The population density of E. huxleyi is restricted by Nucleocytoviricota viruses, including E. huxleyi virus 201 (EhV-201). Here, we show that the dsDNA genome inside the EhV-201 virion is protected by an inner membrane, capsid, and outer membrane. Virions of coccolithoviruses are unique within the family Phycodnaviridae because they contain not only a membrane inside the capsid but also an additional membrane wrapped around the outer capsid surface, similar to the African swine fever virus from the family Asfaviridae. EhV-201 virions infect E. huxleyi by using fivefold vertices to bind to and fuse the virus’ inner membrane with the cell plasma membrane.

(F) AlphaFold2-predicted structure of EhV-201 major capsid protein with double jelly roll fold. The jellyroll cores J1 and J2 are each composed of two β sheets named according to the convention BIDG and CHEF. The transmembrane proteins from the EhV-201 outer membrane bind to the capsid; however, there are additional interactions between the major capsid proteins and the outer membrane. The loop is predicted to form helices α3 and α4, which are 13- and 20-residue long, respectively, and are positioned at the outer surface of the capsid. Fitting the predicted EhV-201 capsomer structure into the sub-tomogram reconstruction of the virion vertex positions helices α3 and α4 inside densities connecting the capsid to the outer membrane. Therefore, we speculate that the amphipathic helices attach the outer virion membrane to the capsid. The abundant capsid-outer membrane contacts may enable EhV-201 virions to withstand deformation without negatively affecting the infectivity of the virus. The reconstruction, because of its limited resolution, did not enable identification of minor capsid proteins mediating contacts between the inner membrane and the capsid, as is the case in other NCVs such as Tokyovirus, PBCV-1, and African swine fever virus.

>[18x]MSGFGGGSSGAGSLTQLLATGSMDAALTQNATRTFWKSSYQKHSLFALESINQPFTTQVQFGAESHITVNRQGDLLSWMYLKIVLPGLKVQNQADTVQPTQQSFASLDNDVAAQADVSHVLPYIEGAYTEASLNTKEQLIAEAKNSYEAAKYNAAPLPVAAQMQSTEMPDFDYAYWTEAIGFHLIKRAEFKVGGATIDTIWSELLFAMEELMGRAGRRLTETIGRTLRRPTELMKASRQEQILYVPLPWYFTKHPSLAFPLVAATYHNIQLWVQWAQLNSCIIKSRSNLVVLHAERNVPISDDHLRASLECTYVHLEAAERDALTANAGTQLIVQHQAHLQQVSSNNVTARLNFNFPVLEFYYFLRRKANKDAGDHFNFSGIGGRDPVVSAELLFNNTARVTQKPAVWWRAVQALQFHSSAPLTNIYSYSFSLSPEDPITPSGSANFSRLDSVELALTLQDDFGAAHDANSELFVFARSYNILKFTNGLAGLLYSN;> MPSIAFSGISTKPGELEFHVPSVLSKHNRAGLLKSIDFPYSQRTIESSWNKLHYMESIRITPESRSVSVLLTDKESGDRVEMLAMVPLTTNKIIEISTATTDGTIILVTEEPHGFFAPGCFGKEVRNVISSYKSIFPHGTPPFILIHGSNGSVQVDPALFEYNDEYSVKIKYTAIRTEFKLFGKGDHGWMVTPEFPTISMLCQVITNAMNSAIIFNHDDPAARTRMYPGTCSNTHVIESVSGDSLAKALLGYDGVYAGWEEITIPAGMYCYGELDLSKMIAAKMNRWHIDRESSIIFRGVSGYTWNVTLPSGNYGTPEKLAHCIQHMMNMTAKNRKNPYCVRFTLNEGSSHRGKFVFVAAEPFDLLFGDDESIDPSILGFEPVDHIGRNSYMSENDLGAPLMKPNCNVYDVDEIPGTHQIRIGRRTRLAVDGKIRGYSGGTLRLNTVNRTTGAPKCHGMNKGDVVTLTTVMPAPDGATGTKREGFTFRAKNKIMGVVVADENENPDASSLHVSVPSMSWTLGIGSYITIDSQAAPISVALFDPGKNQFFRDSIGASRLGFSNGVSTGQHGVVVSQCAVNLEPRTVDVSFIEGSMTSASTEMYNQNGKSLITQVPSDRSSGPVPQGMVRFNNALQQFKLEFTNPDGSPYHFNHASLSLLMEFDD>[4x]STVELCGQWDTRTVAGGR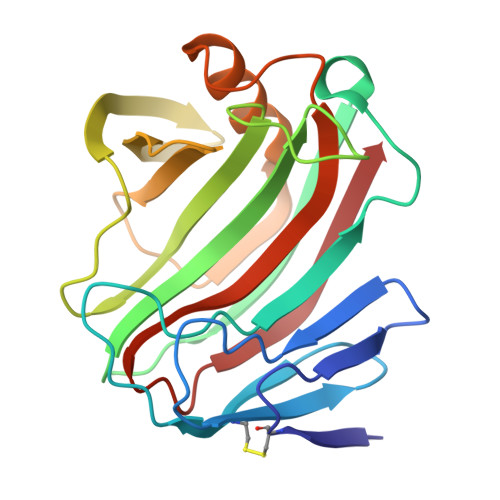YTVSNNVWGAETAQCIEVGLETGNFTITRAEHDNGNNVAAYPNIQFAIPQPRRVQELSDVRTSWTLTPITTGRWNAAYDIFFAANPNHVTYSGDAELMIWLNKNGDVMPIGSRVATVELAGATWEVWYADNGAMNVISYVRTTPTTSVTELDLKAFIDDAVARGYIRPEWYLLSVQTGFELFTGGAGLRSADFSVTVQ>MLAVGIVGLPNVGKSTLFNALTRANALAANY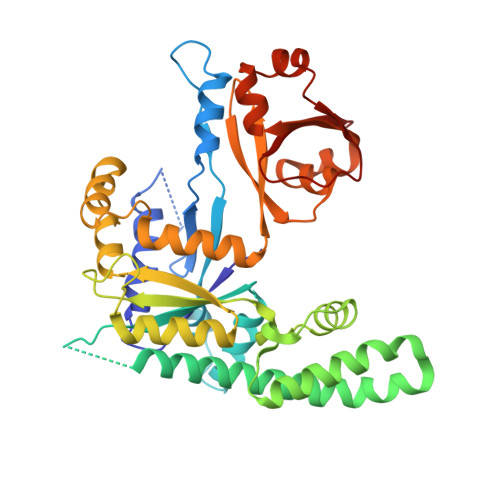PFATIDKNVGVVPLEDERLYALQRTFAKGERVPPVVPTHVEFVDIAGLVKGAHKGEGLGNQFLAHIREVAAIAHVLRCFPDPDVVHVMGRVDPLEDAEVVETELLLADLATLERRLERLRKEARADRERLPLLEAAEGLYVHLQEGKPARTFPPSEAVARFLKETPLLTAKPVIYVANVAEEDLPDGRGNPQVEAVRRKALEEGAEVVVVSARLEAELAELSGEEARELLAAYGLQESGLQRLARAGYRALDLLTFFTAGEKEVRAWTVRRGTKAPRAAGEIHSDMERGFIRAEVIPWDKLVEAGGWARAKERGWVRLEGKDYEVQDGDVIYVLFNA[2x]(1R,3S,4R)-1-azabicyclo[2.2.2]octan-3-yl 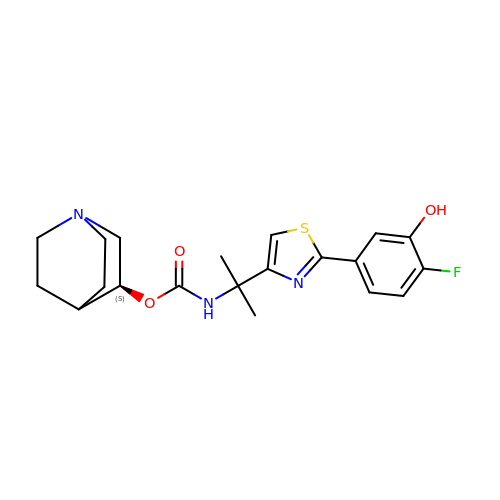{2-[2-(4-fluoro-3-hydroxyphenyl)-1,3-thiazol-4-yl]propan-2-yl}carbamate | C20 H24 F N3 O3 S | LRJXHGILPIXDQG-MRXNPFEDSA-N>[2x]MKKKGSVVIVGRINLSGDTAYAQQTRGEEGCQETSQTGRDKNQVEGEVQIVSTATQTFLATSINGVLWTVYHGAGTRTIASPKGPVTQMYTNVDKDLVGWQAPQGSRSLTPCTCGSSDLYLVTRHADVIPVRRRGDSRGSLLSPRPISYL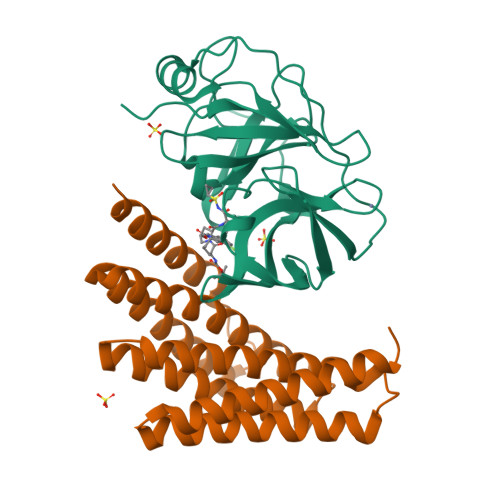KGSAGGPLLCPAGHAVGIFRAAVSTRGVAKAVDFIPVESLETTMRSP;>[2x]SSDEEEARELIERAKEAAERAQEAAERTGDPRVRELARELKRLAQEAAEEVKRDPSSSDVNEALKLIVEAIEAAVDALEAAERTGDPEVRELARELVRLAVEAAEEVQRNPSSSDVNEALHSIVYAIEAAIFALEAAERTGDPEVRELARELVRLAVEAAEEVQRNPSSRNVEHALMRIVLAIYLAEENLREAEESGDPEKREKARERVREAVERAEEVQRDPSGWLNH>CGC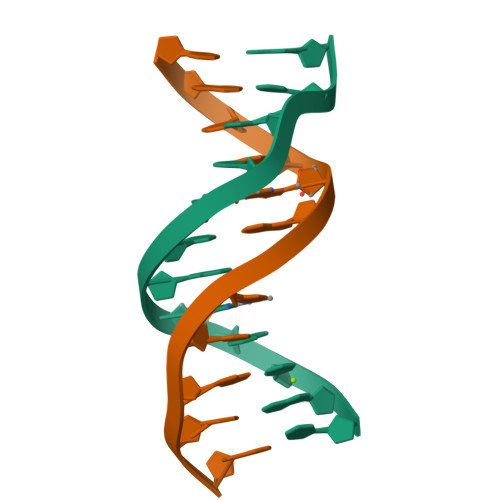GAATCCGCG[2x]>[2x]MSGMKKLYEYTVTTLDEFLEKLKEFILNTSKDKIYKLTITNPKLIKDIGKAIAKA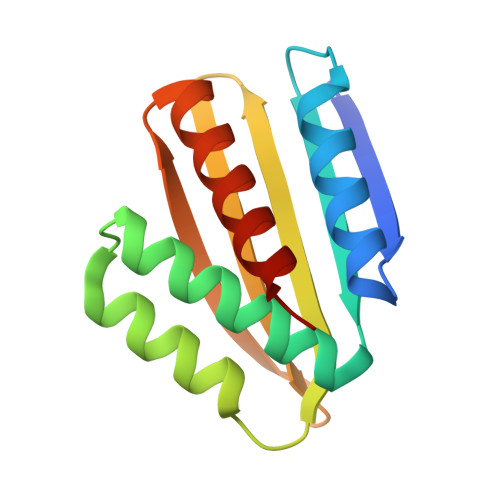AEIADVDPKEIEEMIKAVEENELTKLVITIEQTDDKYVIKVELENEDGLVHSFEIYFKNKEEMEKFLELLEKLISKLSGS>MGHHHHHHRNYHLFEKVRKWAYRAIRQGWPVFS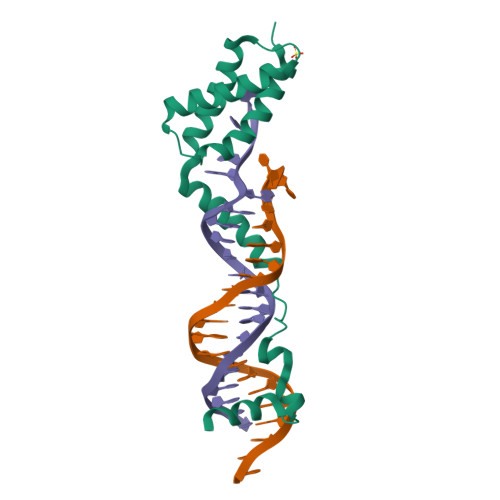QWLDAVIQRVEMYNASLPVPLSPAECRAIGKSIAKYTHRKFSPEGFSAVQAARGRKGGTKSKRAAVPTSARSLKPWEALGISRATYYRKLKCDPD[2x]> MPELPEVETIRRTLLPLIVGKTIEDVRIFWPNIIRHPRDSEAFAARMIGQTVRGLERRGKFLKFLLDRDALISHLRMEGRYAVASALEPLEPHTHVVFCFTDGS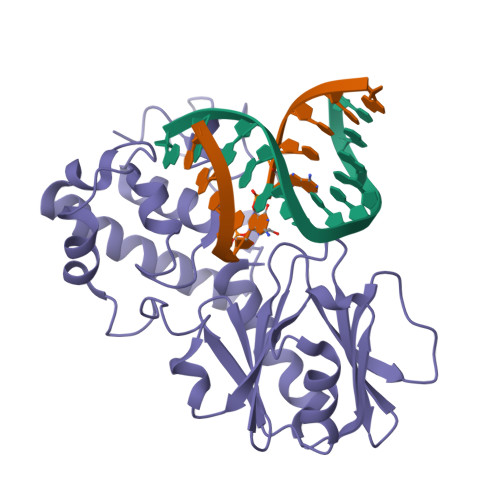ELRYRDVRKFGTMHVYAKEEADRRPPLAELGPEPLSPAFSPAVLAERAVKTKRSVKALLLDQTVVAGFGNIYVDESLFRAGILPGRPAASLSSKEIERLHEEMVATIGEAVMKGGSTVRTYVNTQGEAGTFQHHLYVYGRQGNPCKRCGTPIEKTVVAGRGTHYCPRCQR> GSHDLGAPQNPNAKAAGSRKIHFNWLPPSGKPMGYRVKYWIQGDSESEAHLLDSKVPSVELTNLYPYCDYEMKVCAYGAQGEGPYSSLVSCRTHQEVPS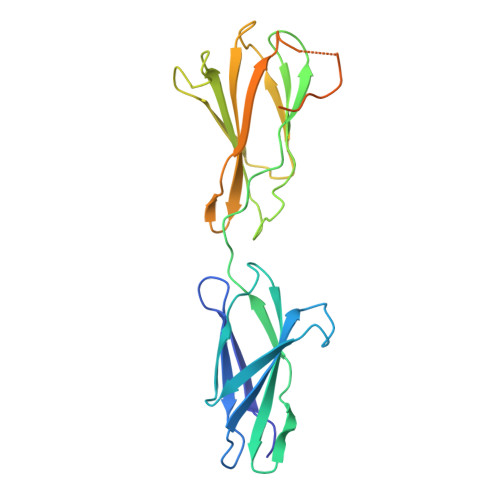EPGRLAFNVVSSTVTQLSWAEPAETNGEITAYEVCYGLVNDDNRPIGPMKKVLVDNPKNRMLLIENLRESQPYRYTVKARNGAGWGPEREAIINLATQPKRPMSIPIIPDIPIVDAQSGEDYDSFLMYSDDVLRSPSGSQRPSVSDDTE> MDNNKAEADTSSSMADPETRPTYTTHHLAIPSGV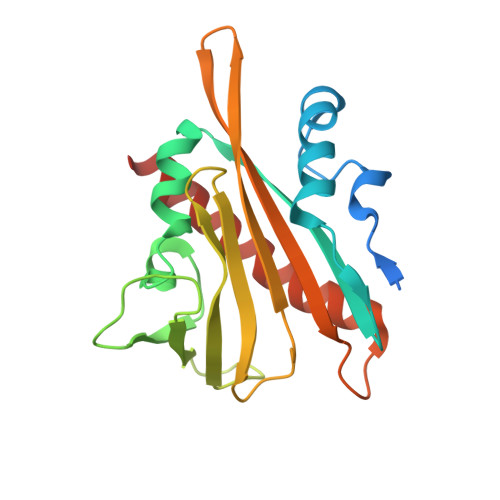TQDEFDELKQSVVEFHTYQLSQNQCSSLLAQRIRAPNDVVWSIVRRFDQPQTYKHFIKSCSVSDNFTMAVGSTRDVNVISGLPAATSTERLDILDDDRQVTGFSIIGGEHRLRNYRSVTSVHGFNRDGAICTVVLESYVVDVPEGNTEEDTRLFADTVVKLNLQKLVSVAESQVI>[2x]SFQEQ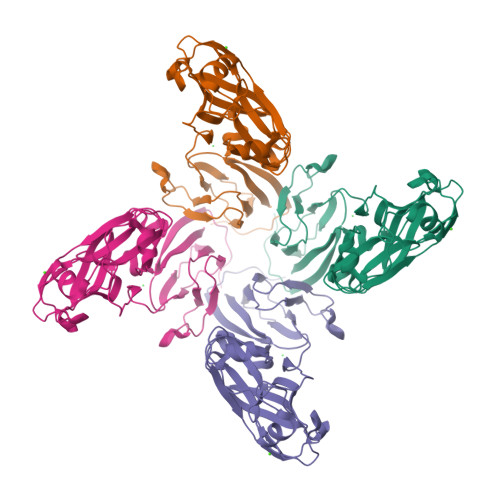TTKSRDVNSFQIPLRDGVRELLPEDASRNRASIKSPVDIWIGGENMTALNGIVDGGRKFEAGQEFQINTFGSVNYWVSDEEIRVFKEYSARAKYAQNEGRTALEANNVPFFDIDVPPELDGVPFSLKARVRHKSKGVDGLGDYTSISVKPAFYITEGDETTDTLIKYTSYGSTGSHSGYDFDDNTLDVMVTLSAGVHRVFPVETELDYDAVQEVQHDWYDESFTTFIEVYSDDPLLTVKGYAQILMERT>[2x]GPLGSKRVIVIGGALAETAFALGGAETPRYRLVGADTTCTYPDAAKRLPKVGYQRALSAEGLLSLRPDLVLASAEAGPPTAIAQVKGAGVTVT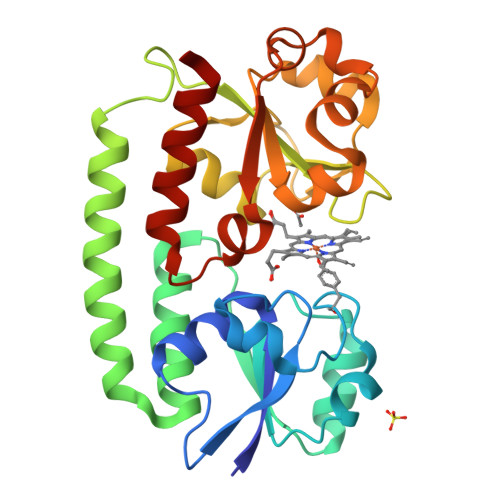TFDERHDVESVRAKITGVAQALDVRDAGAALLQRFDRDWQAARDAVAARVPGGAQPPRVLFVLNHTGTQALVAGQRTAADAMIRYAGARNAMQGFDHYKPLTTEALAAAAPDVVLISDEGLAAVGGHAALLATPGFGATPAGRARRVVSLDALFLLGFGPRLPLAVTTLHRRLSDALA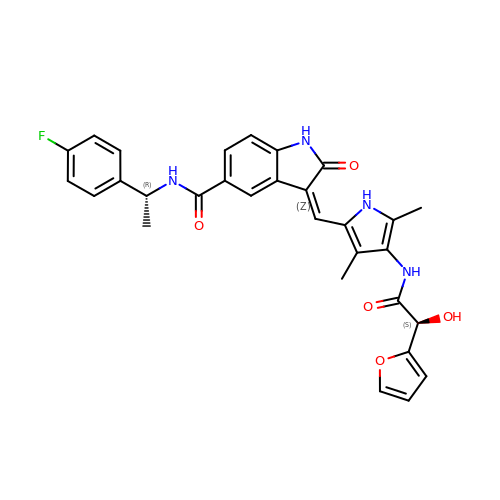(3Z)-N-[(1R)-1-(4-fluorophenyl)ethyl]-3-[(4-{[(2S)-2-(furan-2-yl)-2-hydroxyacetyl]amino}-3,5-dimethyl-1H-pyrrol-2-yl)methylidene]-2-oxo-2,3-dihydro-1H-indole-5-carboxamide | C30 H27 F N4 O5 | XSBCFLGDNDHVIP-ZQAWARHGSA-N(3AS,4R,5S,8AS,8BR)-4-[5-(5-CHLOROTHIOPHEN-2-YL)-1,2-OXAZOL-3-YL]-2-[3-[1-(2-HYDROXYETHYL)PYRROLIDIN-1-IUM-1-YL]PROPYL]-4,6,7,8,8A,8B-HEXAHYDRO-3AH-PYRROLO[3,4-A]PYRROLIZINE-1,3-DIONE 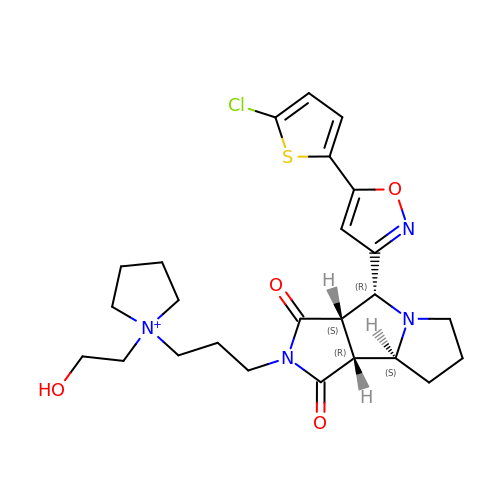| C25 H32 Cl N4 O4 S | NGWQPUFWVMNLQW-ZMVGRULKSA-N[[(2E)-2-[[4-[(E)-[[azaniumylidene(azanyl)methyl]hydrazinylidene]methyl]phenyl]methylidene]hydrazinyl]-azanyl-methylidene]azanium 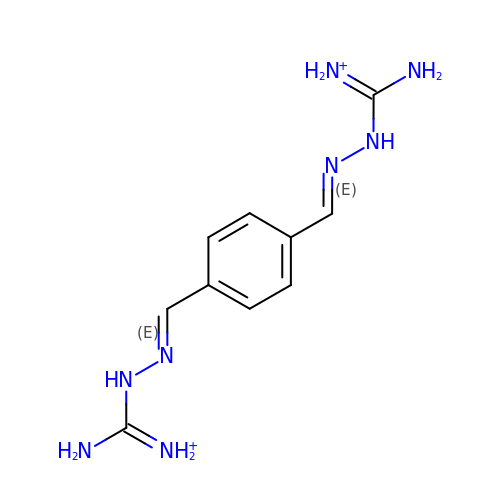| C10 H16 N8 | DJQYBCUFGZTQSR-IAGONARPSA-P N-({1-[(2S)-2-carboxy-4-phenylbutyl]cyclopentyl}carbonyl)-L-tryptophan | C28 H32 N2 O5 | 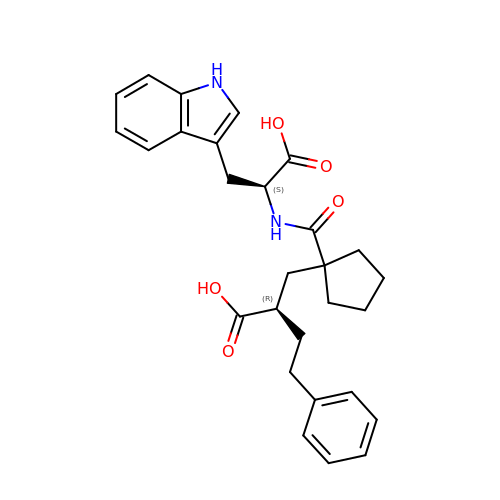MPZIROHQGMKFGS-YKSBVNFPSA-N> QDKIEALSSKVQQLERSIGLKDLAMADLEQKVLEMEASTYDGVFIW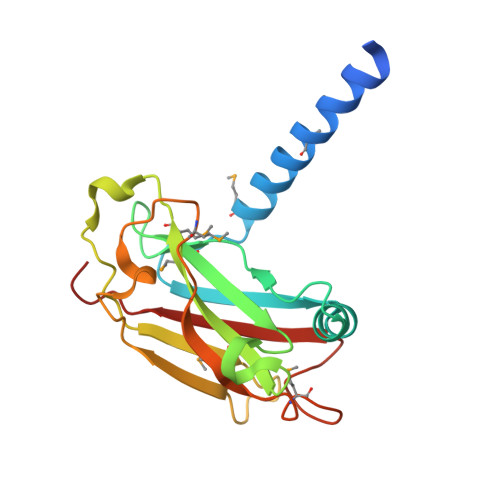KISDFARKRQEAVAGRIPAIFSPAFYTSRYGYKMCLRIYLNGDGTGRGTHLSLFFVVMKGPNDALLRWPFNQKVTLMLLDQNNREHVIDAFRPDVTSSSFQRPVNDMNIASGCPLFCPVSKMEAKNSYVRDDAIFIKAIVDLTGL> TLSILVAHDLQRVIGFENQLPWHLPNDLKHVKKLSTGHTLVMGRKTFESIG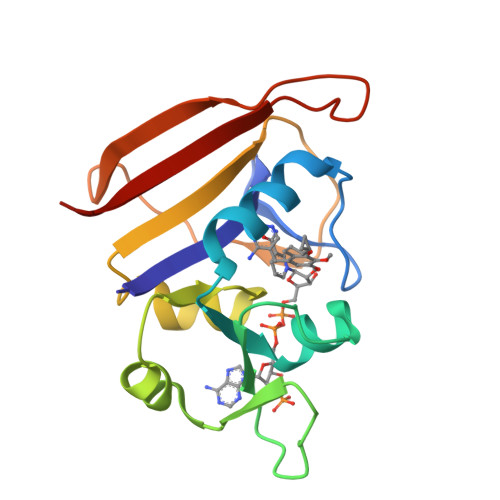KPLPNRRNVVLTSDTSFNVEGVDVIHSIEDIYQLPGHVFIFGGQTLYEEMIDKVDDMYITVIEGKFRGDTFFPPYTFEDWEVASSVEGKLDEKNTIPHTFLHLIRKK4-{2-[(cyclopentylmethyl)amino]ethyl}-2-(methylamino)-3,7-dihydro-8H-imidazo[4,5-g]quinazolin-8-one | C18 H24 N6 O | 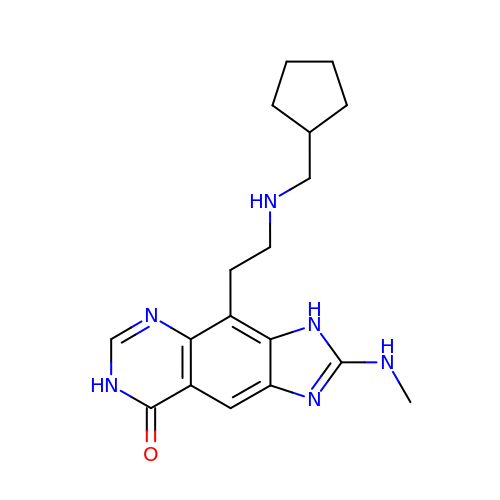IEHXPXUWCFKZTR-UHFFFAOYSA-N>GSHMDKNGEIVEKIKDEKSINQNLDFLRNYRDSYNRTPLMVACMLGMENAIDKLVENFDKLEDKDIEGSTALIWAVKNNRLGIAEKLLSKGSNVNTKDFSGKTPLMWSIIFGYSEMSYFLLEHGANVNDRNLEGETPLIVASKYGRSEIVKKLLELGADISARDLTGLTAEASAR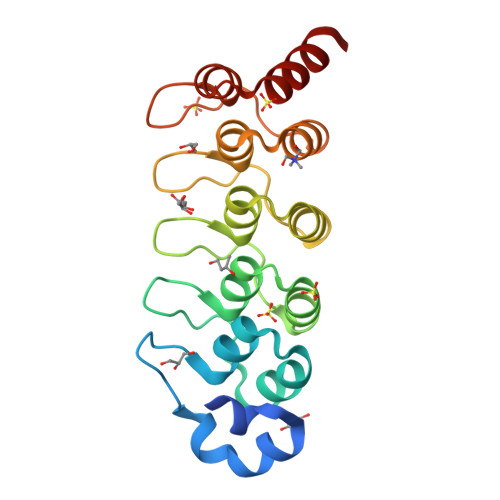IFGRQEVIKIFTEVRRA[2x]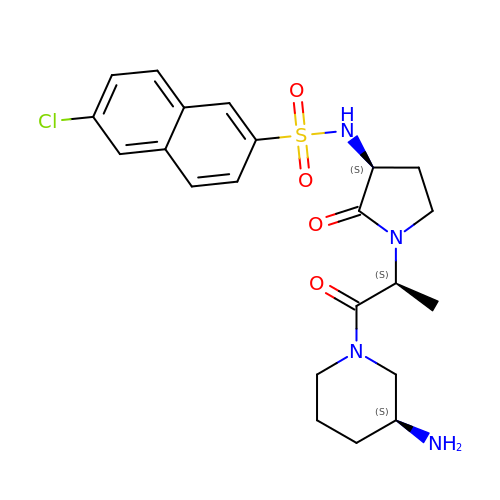N-[(3S)-1-{(2S)-1-[(3S)-3-aminopiperidin-1-yl]-1-oxopropan-2-yl}-2-oxopyrrolidin-3-yl]-6-chloronaphthalene-2-sulfonamide | C22 H27 Cl N4 O4 S | SWAVCKCAPZVXAE-DCPHZVHLSA-N>[3x]MQGDAKVIEYLNAALRSELTAVSQYWLHYRLQEDWGFGSIAHKSRKESIEEMHHADKLIQRIIFLGGHPNLQRLNPLRIGQTLRETLDADLAAEHDARTLYIEARDHCEKVRDY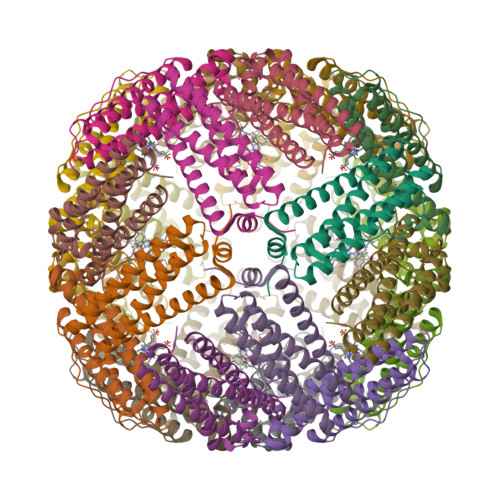PSKMLFEELIADEEGHIDYLETQIDLMGSIGEQNYGMLNAKPADEAE>[2x]SHAAILWNEAKAFIAECYAELGKAEEVADRLDSIKSEIDLTGSYVHTKEELEHGAKMAWRNSNRCIGRLFWNSLNVIDRRDVRTKEDVRDALFHHIETATNNGKIRPSITIFPPEEKGEKQVEIWNHQLIRYAGYEAAGEAIGDPASCSLTAACEQLGWRGERTDFDLLPLIFRMKGDEQPVWYELPRSL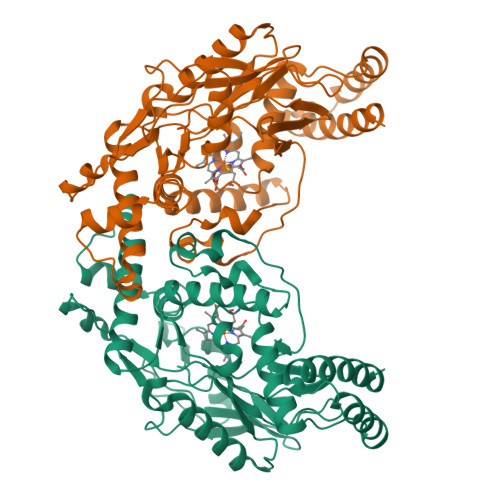VIEVPITHPDIEAFSDLELKWYGVPIISDMKLEVGGIHYNAAPFNGWYMGTEIGARNLADEKRYDKLKKVASVIGISTNYNTDLWKDQALVELNKAVLYSYKKQGVSIVDHHTAASQFKRFEEQEEEAGRKLTGDWTWLIPPISPAATHIFHRSYDNSIVKPNYFYQDKPYE> XPLVVAASIIAILHL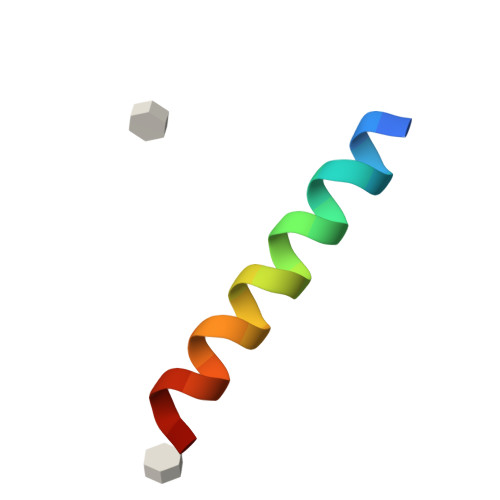ILWALDRLX> ALMITDECINCDVCEPECPNGAISQGDETYVIEPSLCTECVGHYETS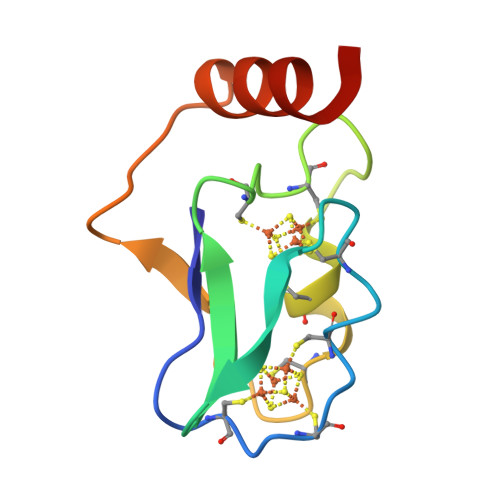QCVEVCPVDCIIKDPSHEETEDELRAKYERITGEG The lasso peptide MS-271 is a ribosomally synthesized and post-translationally modified peptide (RiPP) consisting of 21 amino acids with D-tryptophan at the C-terminus, and is derived from the precursor peptide MslA. MslH, encoded in the MS-271 biosynthetic gene cluster (msl), catalyzes the epimerization at the Cα center of the MslA C-terminal Trp21, leading to epi-MslA. Herein, based on X-ray crystallographic studies in association with MslA core peptide analogues, we show that MslH is a metallo-dependent peptide epimerase with a calcineurin-like fold. The crystal structure analysis, followed by site-directed mutagenesis, docking simulation, and ICP-MS studies demonstrate that MslH employs acid/base chemistry to facilitate the reversible epimerization of the C-terminal Trp21 of MslA, by utilizing two pairs of His/Asp catalytic residues that are electrostatically tethered to a six-coordination motif with a Ca(II) ion via water molecules.

In the mutagenesis studies, all residues except for His295 were substituted with alanine, while His295 was substituted with asparagine, with the same size as histidine, because of the instability of the His295A variant during the purification and enzyme reaction. The in vitro experiment revealed that all variants lacked epimerase activity, indicating that the four residues are crucial for catalysis. In contrast, the loss of catalytic activity of the His295N and Asp11A variants could be due to a structural collapse of the metal-binding and substrate-binding sites, caused by a breakdown of the hydrogen bonding network between six-coordination motif and Asp11/His295 via the w2 water molecule and substrate. Therefore, we evaluated the His295N and Asp11A variants from a structural aspect. We obtained their crystal structures, MslH Asp11A:apo and MslH His295N:apo at 2.41 and 2.55 Å resolutions, respectively. Both crystal structures indicated that the variants retained the same six-coordination motif as that in the wild-type MslH crystal structure. The His295N substitution had no effect on the active center organization, while the Asp11A substitution led to the flexibility of His295 in the MslH Asp11A:apo crystal structure, where a 1:1 alternative state was observed for the His295 residue. Moreover, the comparison of the MslH His295N:apo structure with the MslH:MslA Trp21G complex structure showed that the distance between the Cα center of MslA Gly21 and Oδ of Asn295 atom is 4.5 Å, which is longer than that (3.4 Å) in the MslH:MslA Trp21G structure. These observations suggested that the Asp11 and His295 residues would play important roles in maintaining the appropriate catalytic state of MslH.

> MTRLTVALSGDCMVTRGGLITSDPAAERLRDLLRGTDFAVTNLEVVPSDGRGHPVHNAVGGGCLIADSAVLDEVTAAGFSVLGCANNHAMDLGTEGVLGTMDLLRARGIPYAGIGADLTGARRPVYADRPGGSLALLSCTATFLPGQEAADPSPELPGRPGLNPLRHTATMQVTADQMDVLRTIDAETGLRARRAEARALLGVDPALLGPDRLALFGTRFRTADAPGFTTECDPRDLDEIARWVGEARLRADLVVVSVHSHEPGPTPETPGEFLRVFAHRMIDEGAHAVVGHGPNFLRGVELYRNKPIFYSLGNIVSQIELTDRVSAEDYAKVTAERPLTPGRYYDRLSGHGTRLFAPHRRYWQSLVPVLTFEDGTLTAARLHPVDLGFGRPVHRRGRPRLADRAEAEKTLTDVAQLSQPYGTAIEVMDDGTGELALDVA>GSPSDNSGAEEMEVSLAKPKHRVTMNEFEYLKLLGKGTFGKVILVKEKATGRYYAMKILKKEVIVAKDEVAHTLTENRVLQNSRHPFLTALKYSFQTHDRLCFVMEYANGGELFFHLSRERVFSEDRARFYGAEIVSALDYLHSEKNVVYRDLKLENLMLDKDGHIKITDFGLCKEGIKDGATMKTFCGTPEYLAPEVLEDNDYGRAVDWWGLGVVMYEMMCGRLPFYNQDHEKLFELILMEEIRFPRTLGPEAKSLLSGLLKKDPKQRLGGGSEDAKEIMQHRFFAGIVWQHVYEKKLSPPFKPQVTSETDTRYFDEEFTAQMITITPPDQDDSMECVDSER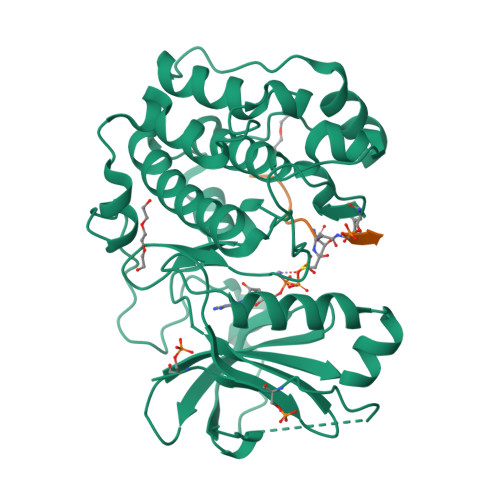RPHFPQFSYSASGTA[2x];>[2x]GRPRTTXFAE>[2x]MGILKTLSAPIILENSNSTFTFLPGGDNFEWIHESIMINAFQGNTLDGSTNNLYLRIYKDNSLAFYPLIGMNSKSTIKSGTSTLIFEGTAEDISYTVTFRLTPYGIWFWDISLSGNCNKADIIYSQDIGVGTKGSVNSNELYLAQYLGHSIFQGDYGYVICSRQNMAQGDLFPYLQQGSLGIRSIAYSTDGTQFFGLSYKKTNIPEALYGDLPSKNKQYELAHTALQTEAFSLSGTKQFSFYGICKTNHPEVIREIEYIQELEKAYAYHESGEILPVNVPTLQNIGAPYASSRWDAKQVEHYFPKRLLEEKEEEALLSFFTPEKSHVVLQDKELTTERPHGHILMTNFDVTKVPQGVVSSTNYMYGAFNCQFVVGNTTYNKLLSNHRGLLNIQKDSGQRIFIKIGDCYRQLTLPAAYEMNVAGSTWYYQLDEDVLIITSFAMYNRPEIVLKVQSLGHKKYDFIVTHQLTVGPNEYENEIKLTREGNIL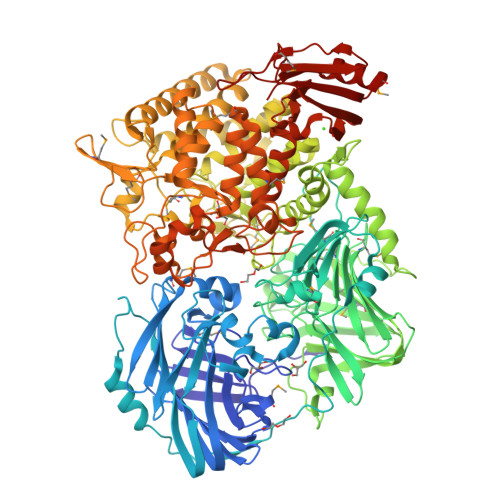QLSPTDPVVTNHFYPELSFRMRIPEDCTLSDDSIFFHNNTTINPSLLSIEILQKSSFDIVMQGFDTGNVIPFLDQYDYKEQLEAYRIYYDQLVCNFKLSAPDKIPLSAEKLNAIIHWYAHDALIHFASPHGLEQSGGAAWGTRDVCQGPIEFFLTTGHFDLVRHILITLYSHQIEGGFEWPQWFMFDHYPIHQEDCHGDVVFWPLKAISDYIQATGDTSILNELVDYRTAKDALPTNQPETILIHIKRAVTTIKNRYLSGTALISYAGGDWDDTLQPANSELKENLVSAWTQALAEQTLELLCSAIKGIDHDFSKELSHMANDIRTSFYQYLIKDGVIAGFLYRESEEHMKYMLHPDDTESSIHYRLLPLTRSIIAQLADFKLATRNLEIIDEHLACPDGVRLMDHPASYSGGISKIFLRAEQAANVGREISLQYVHAHIRYIEALATMGLSKKAWDALMRINPILLTDYVPNALTRQSNVYFSSSEGCFDDRYEYAKNFDKLRTGDINVKGGWRLYSSGPGIYIRRIIADLLGIRFGHNVIHIDPVVTKELDGVTLQFTCFGKTVFFTYHVDDTMDKHICVKSNNNILPGDNLNNIYRDGGIQIAKDVFLSAAMSDNNFHIYVKNLEHHHHHH>MAHHHHHHVDDDDKMTMASTPASRYITDMTIEELSRDWFMLMPKQKVEGPLCIRIDQAIMDKNIMLKANFSVIF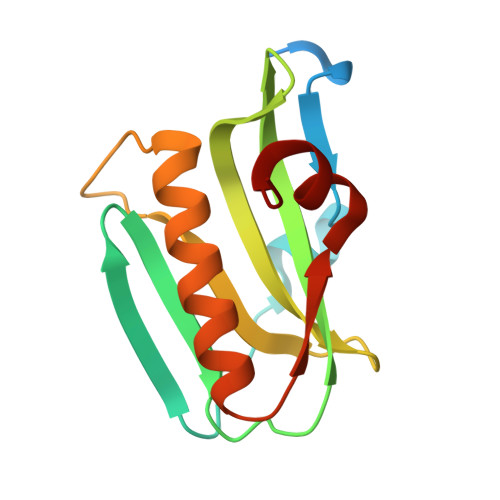DRLETLILLRAFTEEGAIVGEISPLPSFPGHTIEDVKNAIGVLIGGLEANDNTVRVSKTLQRFAWGS[2x]> GMAIAPQQIQERLKQEQYQKFVVADIGNFPHCLAQTPEGIASGQRYQKYSTNSLSRTPPFSQWGAPQLLTPKSAQEYIKFAQQRNKKSSFKIDGEAVRVSECSNFAYHSAGVLLDDPQIRTQYDVAVIGSMHSNGRYLHNITLLVPKGSRLPQPPEQLTAEVFPIGTLIVDPWAVGMGHPPEQALAIPKEQFAYNRSLFPATVNYQSALDESLTSTRTGQLTPYTGTPS

Among all bacterial pathogens, Legionella pneumophila maintains the largest known set of translocated substrates, delivering over 300 proteins to the host cell via its Type IVB, Icm/Dot translocation system. In at least nine instances, this regulation is direct—a hallmark of an emerging class of proteins called metaeffectors, or “effectors of effectors”. Through detailed structural and functional analysis, we show that metaeffector activity derives from a diverse range of mechanisms, shapes evolution, and can be used to reveal important aspects of each cognate effector's function. After release into the host cell, translocated bacterial substrates (effectors) regulate one another through several different functional interactions: indirectly, through counteracting modification of a shared host target, or directly through either steric complex formation or direct modification of one effector by another.

To define the mechanism of LegL1 inhibition of RavJ, we first solved the crystal structure of the N‐ and C‐terminal portions of RavJ spanning amino acid residues 1–228 and 251–371, respectively (Table EV4). Structures for amino acid residues 1–228 and 251–371 of RavJ were solved separately to a resolution of 1.3 and 1.9 Å, respectively. Despite no identifiable sequence similarity, the overall fold of the N‐terminal domain of RavJ resembled that of papain‐like cysteine protease family members. Comparison of RavJ with its top structural homolog, human tissue transglutaminase (TGM2), identified three conserved residues (C101, H138, D170) along with another adjacent residue (W172) as a putative catalytic site. The N‐terminal structure contains a structurally conserved putative catalytic triad (C101/H138/D170). To determine which of these structural elements are essential for effector function, we tested the effect of their ablation on yeast growth. Strikingly, single substitutions in each of the four N‐terminal catalytic site residues, as well as the C‐terminal loop mutant, abrogated the yeast growth inhibition of RavJ. While expression of full‐length RavJ showed a severe growth defect in a spot dilution assay, mutation of each of the putative catalytic residues or the adjacent W172 to alanine fully relieved toxicity as did substitutions in the conserved C‐terminal motif.> QCASSP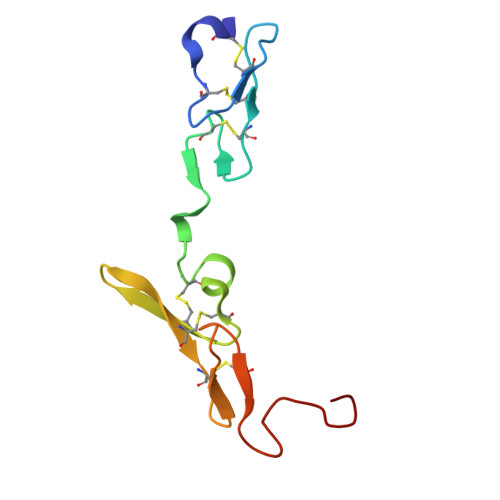CQNGGSCKDQLQSYICFCLPAFEGRNCETHKDDQLICVNENGGCEQYCSDHTGTKRSCRCHEGYSLLADGVSCTPTVEYPCGKIPILE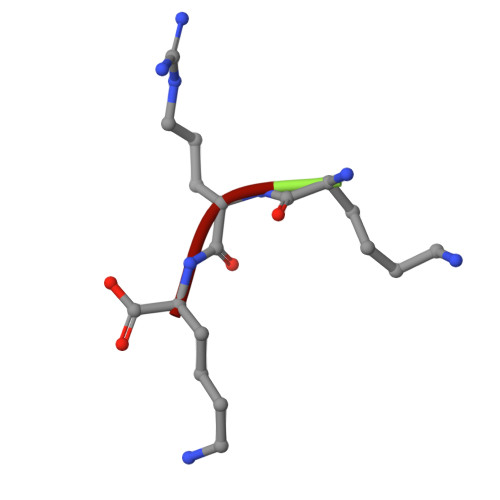> KRK> XWLAQRLGRELRR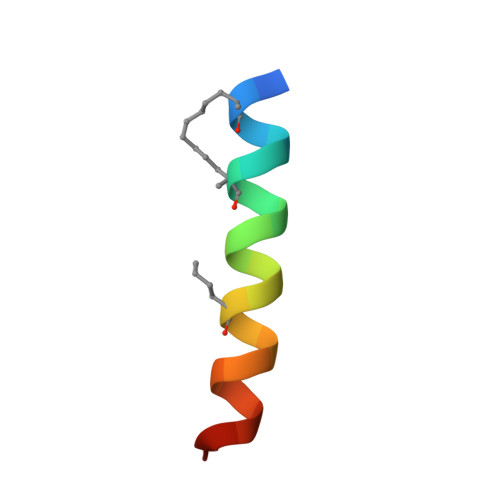LSDEFVDSFK(2R)-2-[[(2S)-2-[[(2R)-2-[(2R,3S,4R,5R,6S)-5-acetamido-3-[(2S,3R,4R,5S,6R)-3-acetamido-6-(hydroxymethyl)-4,5-bis(oxidanyl)oxan-2-yl]oxy-2-(hydroxymethyl)-6-oxidanyl-oxan-4-yl]oxypropanoyl]amino]propanoyl]amino]pentanedioic 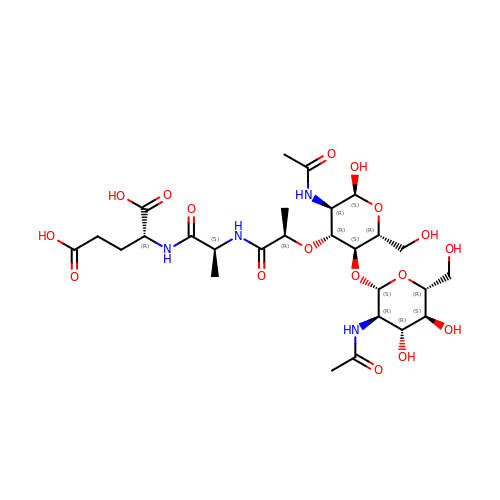acid | C27 H44 N4 O17 | ZIRNZNIZUAXLNB-XNKNRSQBSA-N> HHEADRIPVVLDNPPWAKPFELLVSFLNTPKYGTFDPTPVVPVFFPFWFGMIVGDIGYALLFYLVGRWLSGYVKRNEPLVIDLFALKLKPQVIGKLVHILNWMVFWTVVWGVIYGEFFGTFLEHLGVFGTPEHPGLIPILIHRIDTAKTANLLILLSVAFGVVLVFFGLALRAYLGLKHRHMAHFWEGVGYLGGLVGVLALAASYLGNLQAGWLQGLMYLGFGVFLLAVLMSRIWLMIPEI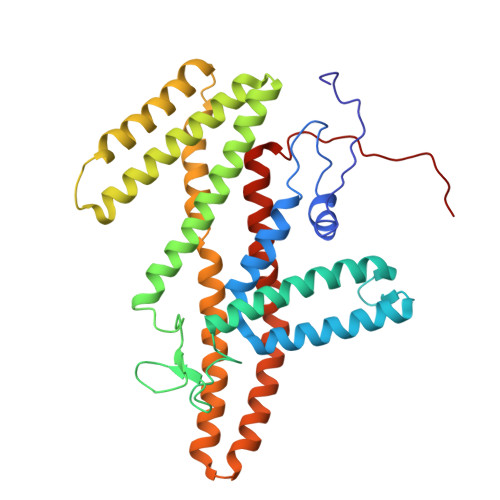FTQAGHILSHIRIYAVGAAGGILAGLLTDVGFALAERLGLLGVLLGLLVAGVLHLLILLLTTLGHMLQPIRLLWVEFFTKFGFYEENGRPYRPFKSVR> YEASILTHDSSIRYLQEIYNSNNQKIVNLKEKVAQLEAQCQEPCKDTVQIHDITGKDCQDIANKGAKQSGLYFIKPLKANQQFLVYCEIDGSGNGWTVFQKRLDGSVDFKKNWIQYKEGFGHLSPTGTTEFWLGNEKIHLISTQSAIPYALRVELEDWNGRTSTADY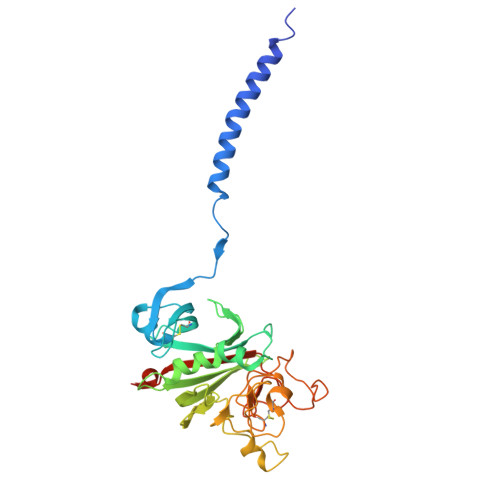AMFKVGPEADKYRLTYAYFAGGDAGDAFDGFDFGDDPSDKFFTSHKGMQFSTWDNDNDKFEGNCAEQDGSGWWMNKCHAGHLNGVYYQGGTYSKASTPNGYDNGIIWATWKTRWYSMKKTTMKIIPFNRLTIGEGQQHHLGGAK> SKKIGLFYGTQ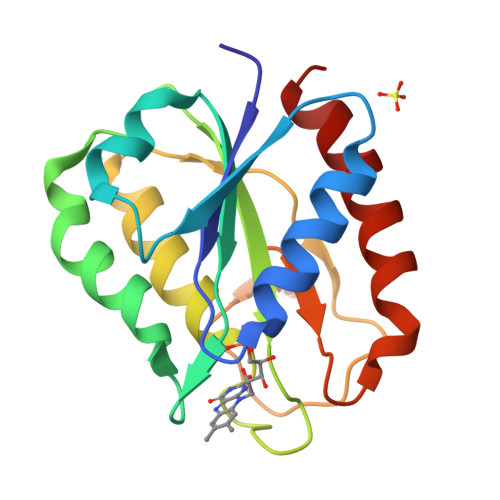TGKTESVAEIIRDEFGNDVVTLHDVSQAEVTDLNDYQYLIIGCPTWNIGELQSDWEGLYSELDDVDFNGKLVAYFGTGDQIGYADNFQDAIGILEEKISQRGGKTVGYWSTDGYDFNDSKALRNGKFVGLALDEDNQSDLTDDRIKSWVAQLKSEFGL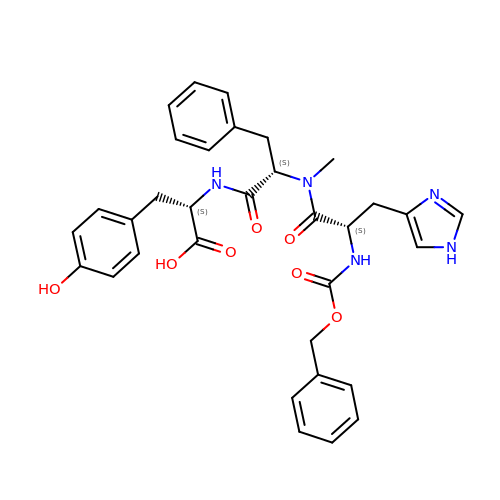N-[(benzyloxy)carbonyl]-L-histidyl-N-methyl-L-phenylalanyl-L-tyrosine | C33 H35 N5 O7 | CPZRYRVSOCXUSE-AWCRTANDSA-N6-fluoro-2-methylimidazo[1,2-a]pyridin-3-amine 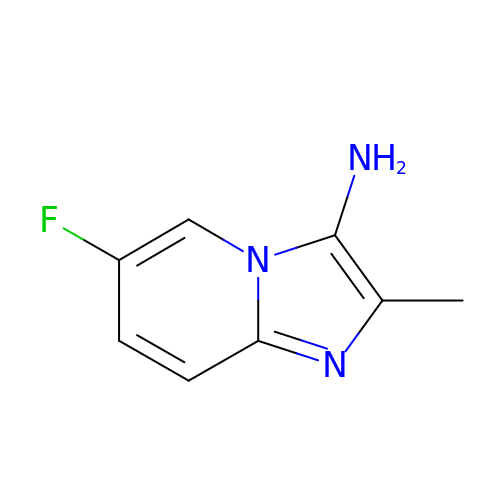| C8 H8 F N3 | OBTLIUIWHZQYAC-UHFFFAOYSA-N1-(4-{methyl[2-({4-[(methylsulfonyl)methyl]phenyl}amino)pyrimidin-4-yl]amino}phenyl)-3-{3-[(4-methylpiperazin-1-yl)carbonyl]phenyl}urea | C32 H36 N8 O4 S | 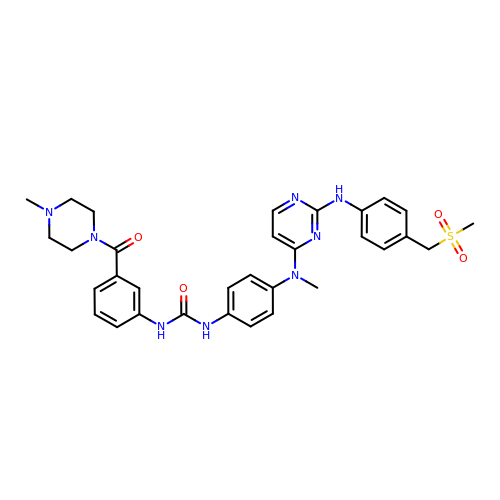HKWWFBIVSCKLOB-UHFFFAOYSA-N> LPLEPNSILGQVGRLLALIGDDINRR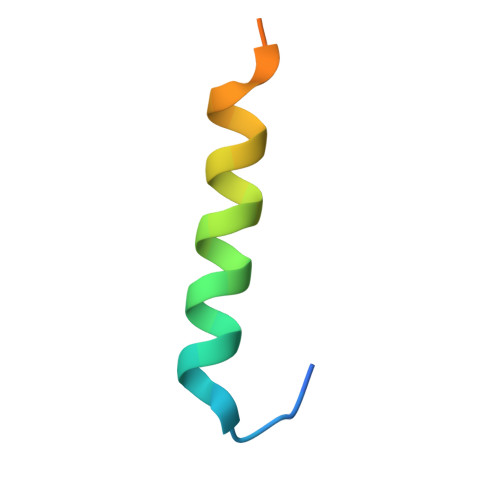YDTEFQNL>[2x]ELDGKAPSHRNLNVQTWSTAEGAKVLFVEARELPMFDLRLIFAAGSSQDGNAPGVAL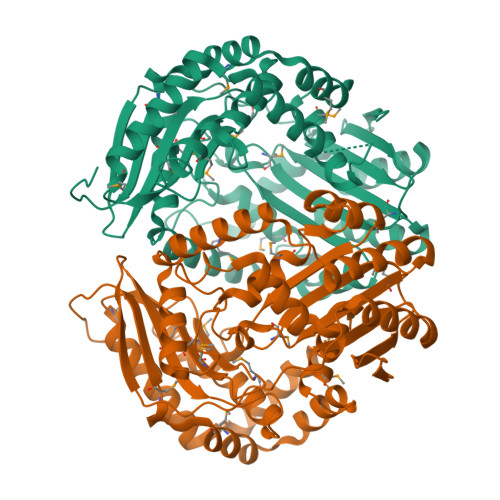LTNAMLNEGVAGKDVGAIAQGFEGLGADFGNGAYKDMAVASLRSLSAVDKREPALKLFAEVVGKPTFPADSLARIKNQMLAGFEYQKQNPGKLASLELMKRLYGTHPYAHASDGDAKSIPPITLAQLKAFHAKAYAAGNVVIALVGDLSRSDAEAIAAQVSAALPKGPALAKIEQPAEPKASIGHIEFPSSQTSLMLAQLGIDRDDPDYAAVSLGNQILGGGGFGTRLMSEVREKRGLTYGVYSGFTPMQARGPFMINLQTRAEMSEGTLKLVQDVFAEYLKNGPTQKELDDAKRELAGSFPLSTASNADIVGQLGAMGFYNLPLSYLEDFMRQSQELTVEQVKAAMNKHLNVDKMVIVSAGPTVAQKPLEHHHHHH>GSMSGNGNAAATAEENSPKMRV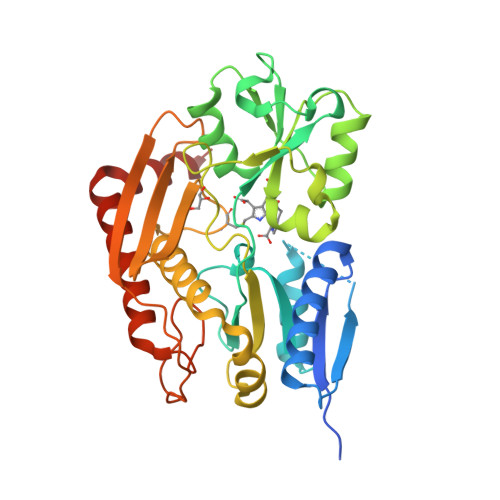IRVGTRKSQLARIQTDSVVATLKASYPGLQFEIIAMSTTGDKILDTALSKIGEKSLFTKELEHALEKNEVDLVVHSLKDLPTVLPPGFTIGAICKRENPHDAVVFHPKFVGKTLETLPEKSVVGTSSLRRAAQLQRKFPHLEFRSIRGNLNTRLRKLDEQQEFSAIILATAGLQRMGWHNRVGQILHPEECMYAVGQGALGVEVRAKDQDILDLVGVLHDPETLLRCIAERAFLRHLEGGCSVPVAVHTAMKDGQLYLTGGVWSLDGSDSIQETMQATIHVPAQHEDGPEDDPQLVGITARNIPRGPQLAAQNLGISLANLLLSKGAKNILDVARQLNDAH[2x]>[2x]MGSSHHHHHHSQDPAEKQKHDGRVKIGHYVLGDTLGVGTFGKVKIGEHQLTGHKVAVKILNRQKIRSLDVVGKIKREIQNLKLFRHPHIIKLYQVISTPTDFFMVMEYVSGGELFDYICKHGRVEEMEARRLFQQILSAVDYCHRHMVVHRDLKPENVLLDAHMNAKIADFGLSNMMSDGEFLRTSCGSPNYAAPEVISGRLYAGPEVDIWSCGVILYALLCGTLPFDDEHVPTLFKKIRGGVFYIPEYLNRSVATLLMHMLQVDPLKRATIKDIREHEWFKQGLPSYLFPEDPSYDANVIDDEAVKEVCEKFECTESEVMNSLYSGDPQDQLAVAYHLIIDNRRIMNQASEFYLASSPPSGSFMDDSAMHIPPGLKPHPERMPPLIADSPKARCPLDALNTTKPKSLAVKKAKWHLGIRSQSKPYDIMAEVYRAMKQLDFEWKVVNAYHLRVRRKNPVTGNYVKMSLQLYLVDNRSYLLDFKSIDDEVVEQRSGSSTPQRSCSAAGLHRPRSSFDSTTAESHSLSGSLTGSLTGSTLSSVSPRLGSHTMDFFEMCASLITTLAR;>MGNTSSERAALERHGGHKTPRRDSSGGTKDGDRPKIL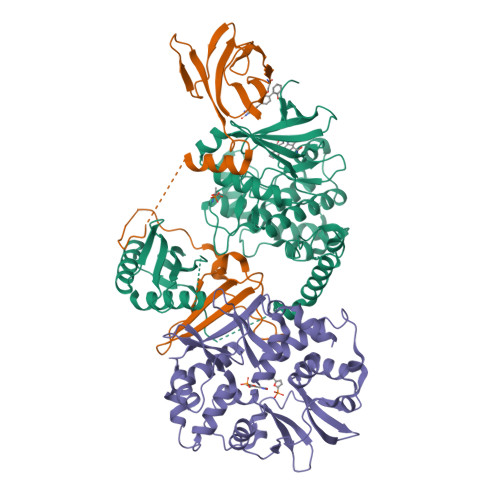MDSPEDADLFHSEEIKAPEKEEFLAWQHDLEVNDKAPAQARPTVFRWTGGGKEVYLSGSFNNWSKLPLTRSHNNFVAILDLPEGEHQYKFFVDGQWTHDPSEPIVTSQLGTVNNIIQVKKTDFEVFDALMVDSQKCSDVSELSSSPPGPYHQEPYVCKPEERFRAPPILPPHLLQVILNKDTGISCDPALLPEPNHVMLNHLYALSIKDGVMVLSATHRYKKKYVTTLLYKPI[2x];>MADLNWETVISSDSSPAVENEHPQETPESNNSVYTSFMKSHRCYDLIPTSSKLVVFDTSLQVKKAFFALVTNGVRAAPLWDSKKQSFVGMLTITDFINILHRYYKSALVQIYELEEHKIETWREVYLQDSFKPLVCISPNASLFDAVSSLIRNKIHRLPVIDPESGNTLYILTHKRILKFLKLFITEFPKPEFMSKSLEELQIGTYANIAMVRTTTPVYVALGIFVQHRVSALPVVDEKGRVVDIYSKFDVINLAAEKTYNNLDVSVTKALQHRSHYFEGVLKCYLHETLETIINRLVEAEVHRLVVVDENDVVKGIVSLSDILQALVLTGGEKKP[2x]>PSAAIYNIDTSSESPDHYLVDHTLDGRVLFPATGYLSIVWKTLARALGLGVEQLPVVFEDVVLHQATILPKTGTVSLEVRLLEASRAFEVSENGNLVVSGKVYQWDDPDPRLFDHPESPTPNPTEPLFLAQAEVYKELRLRGYDYGPHFQGILEASLEGDSGRLLWKDNWVSFMDTMLQMSILGSAKHGLYLPTRVTAIHIDPATHRQKLYTLQDKAQVADVVVSRWLRVTVAGGVHISGLHTESAPRRQQEQQVPILEKFCFTPHTEEGCLSERAALQEELQLCKGLVQALQTKVTQQGLKMVVPGLDGAQIPRDPSQQELPRLLSAACRLQLNGNLQLELAQVLAQERPKLPEDPLLSGLLDSPALKACLDTAVENMPSLKMKVVEVLAGHGHLYSRIPGLLSPHPLLQLSYTATDRHPQALEAAQAELQQHDVAQGQWDPADPAPSALGSADLLVCNCAVAALGDPASALSNMVAALREGGFLLLHTLLRGHPLGDIVAFLTSTEPQYGQGILSQDAWESLFSRVSLRLVGLKKSFYGSTLFLCRRPTPQDSPIFLPVDDTSFRWVESLKGILADEDSSRPVWLKAINCATSGVVGLVNCLRREPGGNRLRCVLLSNLSSTSHVPEVDPGSAELQKVLQGDLVMNVYRDGAWGAFRHFLLEEDKPEEPTAHAFVSTLTRGDLSSIRWVCSSLRHAQPTCPGAQLCTVYYASLNFRDIMLATGKLSPDAIPGKWTSQDSLLGMEFSGRDASGKRVMGLVPAKGLATSVLLSPDFLWDVPSNWTLEEAASVPVVYSTAYYALVVRGRVRPGETLLIHSGSGGVGQAAIAIALSLGCRVFTTVGSAEKRAYLQARFPQLDSTSFANSRDTSFEQHVLWHTGGKGVDLVLNSLAEEKLQASVRCLATHGRFLEIGKFDLSQNHPLGMAIFLKNVTFHGVLLDAFFNESSADWREVWALVQAGIRDGVVRPLKCTVFHGAQVEDAFRYMAQGKHIGKVVVQVLAEEPEAVLKGAKPKLMSAISKTFCPAHKSYIIAGGLGGFGLELAQWLIQRGVQKLVLTSRSGIRTGYQAKQVRRWRRQGVQVQVSTSNISSLEGARGLIAEAAQLGPVGGVFNLAVVLRDGLLENQTPEFFQDVCKPKYSGTLNLDRVTREACPELDYFVVFSSVSCGRGNAGQSNYGFANSAMERICEKRRHEGLPGLAVQWGAIGDVGILVETMSTNDTIVSGTLPQRMASCLEVLDLFLNQPHMVLSSFVLAEKAAAYRDRDSQRDLVEAVAHILGIRDLAAVNLDSSLADLGLDSLMSVEVRQTLERELNLVLSVREVRQLTLRKLQELSSKADEASELACPTPKEDGLAQQQTQLNLRSLLVNPEGPTLMRLNSVQSSERPLFLVHPIEGSTTVFHSLASRLSIPTYGLQCTRAAPLDSIHSLAAYYIDCIRQVQPEGPYRVAGYSYGACVAFEMCSQLQAQQSPAPTHNSLFLFDGSPTYVLAYTQSYRAKLTPGCEAEAETEAICFFVQQFTDMEHNRVLEALLPLKGLEERVAAAVDLIIKSHQGLDRQELSFAARSFYYKLRAAEQYTPKAKYHGNVMLLRAKTGGAYGEDLGADYNLSQVCDGKVSVHVIEGDHRTLLEGSGLESIISIIHSSLAEPRVSVREG[2x]

In mammals, fatty acid synthase (FASN) contains multiple enzymatic domains to catalyse all chemical reactions needed for de novo fatty acid synthesis. An ACP carries substrates from one enzyme to another, sequentially following the chemical reactions. In metazoans, all essential enzymes are included in a single polypeptide chain and are arranged into two main functional domains, each carrying out a key chemical process and named correspondingly the condensing and modifying domains. The entire cycle of fatty acid synthesis requires that ACP carries the substrate from one enzyme to another repeatedly. Here, using a strategy of tagging and purifying endogenous FASN in HEK293T cells for single-particle cryo-electron microscopy studies, we characterized the structural dynamics of endogenous human FASN.

Focusing on these subsets, we refined the condensing and modifying wings separately to high resolutions with the best to 2.5 Å and 2.7 Å, respectively, from the 1,3-DBP sample. From these two separate reconstructions, we generated a composite map of human FASN incubated with 1,3-DBP, in which an ACP is seen bound to the KS domain. This composite map is of sufficient quality for accurate modelling of most of the modifying and condensing wings. For the modifying wing, we also applied symmetry expansion followed by 3D classification to separate particles of the modifying domain into two main categories, with (about 32%) and without (about 68%) well-resolved Ψ-domains attaching to β-ketoreductase (KR). Comparison between the two reveals motions of the Ψ-domains against the rest of the modifying domain, which remains stable. Both KR and Ψ−KR have a Rossmann-like fold, containing two α-helical domains separated by a β-sheet. Indeed, we observed that the β-sheet of KR serves as a hinge allowing progressively increased motion from Ψ−KR towards Ψ−methyltransferase (Ψ−ME). ACP is linked to KR in the modifying wing with a short linker.Phosphatidylinositol 5-phosphate 4-kinases (PI5P4Ks) are emerging as attractive therapeutic targets in diseases, such as cancer, immunological disorders, and neurodegeneration, owing to their central role in regulating cell signaling pathways that are either dysfunctional or can be modulated to promote cell survival. One class of these enzymes, the phosphatidylinositol 5-phosphate 4-kinases (PI5P4Ks), is functionally expressed in mammals to regulate cellular levels of their substrate, PI5P, or generate specific pools of the PI(4,5)P2 product. The role of the PI5P4Ks in response to cell starvation, a process that leads to the negative regulation of mTORC1 activity to initiate autophagy, has also been documented. The regulation of mTORC1 by PI5P4Kγ results in the basal activation of the complex, whereas reduced PI5P4Kγ activity in starvation conditions initiates autophagy. PI5P4Kγ is therefore a target for small molecule inhibition in the context of neurodegenerative diseases.

Compound 40 was selected for crystallography owing to its balance of potency and solubility. The most interesting aspect is the presence of two distinct binding pockets for 40 in PI5P4Kγ that cannot be occupied simultaneously by the ligand. The other three monomer chains (A, C, and D) show the ligand located 18 Å away from the ATP site in a lipid-binding pocket. In this protein conformation, residues Gln378, Tyr379, and Asp380 of the activation loop occupy an inhibitory position in the ATP-binding site. Thus, the binding of 40 into the allosteric pocket appears to stabilize a protein conformation where the activation loop inhibits access to the ATP site. The allosteric binding site in the PI5P4Kγ protein is formed by residues Asp161, Met162, Asn165, Leu166, Tyr169, Leu182, Phe185, Phe272, Leu273, Leu276, Asp374, and Thr377 with the isopropylphenyl moiety of 40 inserted deep into a mostly lipophilic pocket. The pyridine substituent of 40 forms a hydrogen bond with the Thr377 hydroxyl group, and the central pyrimidine ring forms a hydrogen bond with the side chain of Asn165. In chain B, where the ligand occupies the ATP site, the allosteric binding site is occupied by residues Ile375 and Leu376, which form the start of a loop that is mostly missing in PI5P4K crystal structures. In the ATP pocket, the ligand interacts with the Met206 backbone NH through the pyridine nitrogen, not the amino pyrimidine moiety commonly associated with kinase hinge binding. The binding mode of 40 found in chains A, C, and D of the complex fits well with the findings from mutational studies and HDX-MS experiments by Clarke et al. that suggested the putative PI5P-binding site of PI5P4Kγ, not the ATP-binding site, to be the likely region of interaction30 of 1.

>MGHHHHHHENLYFQGHFVQQKVKVFRAADPLVGVFLWGVAHSINELSQVPPPVMLLPDDFKASSKIKVNNHLFHRENLPSHFKFKEYCPQVFRNLRDRFGIDDQDYLVSLTRNPPSESEGSDGRFLISYDRTLVIKEVSSEDIADMHSNLSNYHQYIVKCHGNTLLPQFLGMYRVSVDNEDSYMLVMRNMFSHRLPVHRKYDLKGSLVSREASDKEKVKELPTLKDMDFLNKNQKVYIGEEEKKIFLEKLKRDVEFLVQLKIMDYSLLLGIHDIIRGSEPEEELGPGEFESFIDVYAIRSAEGAPQKEVYFMGLIDILTQYDAKKKAAHAAKTVKHGAGAEISTVHPEQYAKRFLDFITNIFA[4x]> MKMEYLQSEEKKDAINKQIHKKEEKEEKEIKIKRKNKVKQRIQIINQIKKYIEAKQQKKQIQSKNQRKYKGRMINTRKQVFKCLWGAQPAYNFSRIINHLRGDPVYQDNTKDVSLRGTFLRGKYDDLPTMIFFTEACDLTANWIPFFTNPQYDILAHRNVWLLNPRNFGNSDRHPSFDLQEMSDDVMRFMYSQKISMATLGGHGIGGKIALAVGCYHAERVTGVFSIDSSPMDQRYHEAFKEFKGYVNALTEINFKTWSDKDV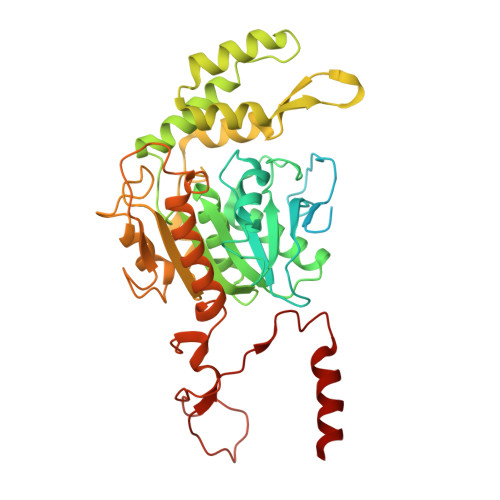KVFLKENIKDPKWRSIFTNNISKNAKTQSDSFNFEINYLNHNLNFNKADSLGNWAVKNGIYTGRAHFIFPEYSRWVHLATNTLPMHKVCARVKGFGHDIFYVQGDENPLNHWVYDFENYANVVASKLNKFLHSYDGVHALLKDRTEIGNFMIPDRIKSRNDSKHIYGDYSPAHLHHNWRFNHIYEKHDELDKKLNEQ> GTALAEMPKRKFTIDDFDIVRPLGKGKFGNVYLAREKQNKFIMALKVLFKSQLEKEGVEHQLRREIEIQSHLRHPNILRMYNYFHDRKRIYLMLEFAPRGELYKELQKHGRFDEQRSATFMEELADALHYCHERKVIHRDIKPENLLMGYKGELKIADFGWSVHAPSLRRRTMCGTLDYLPPEMIEGKTHDEKVDLWCAGVLCYEFLVGMPPFDSPSHTETHRRIVNVDLKFPPFLSDGSKDLISKLLRYHPPQRLPLKGVMEHPWVKANSRRVLP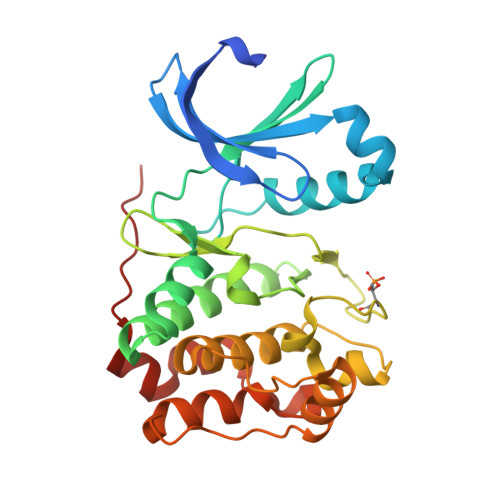PVYQ>[2x]MATGRT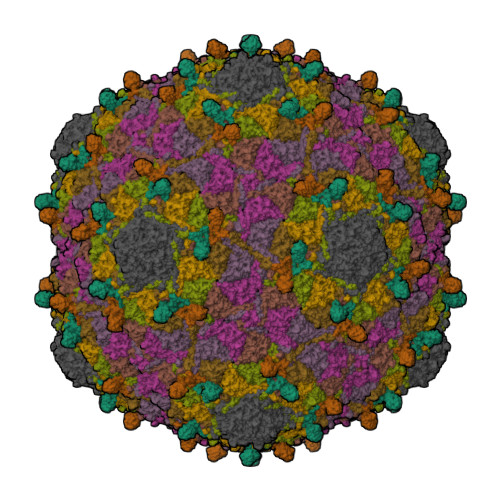TEGRTVTVTTASNTTITGAAGTFVASDVGRTITRAGIPAGTTITAVASGTSATISAAATTSATSAATLGSLNGQSQGLVGWSPETDTEAGAYSVAATNAGTVTPDRLTNAFTPVSQRGRG;>[7x]MGIYRKKDVIPIPYNNLTSRTDAQALIPEEVSKEMLGKATEQSAVLQQFRRIPVGRNQVRFPVLSALPVAYWVNGDTGLKQTTEINWTNKYLNIEEIATIVPVPDNVLADVDVNVWDEAMPYLIEAFGRTLDSAVVFGTNAPGTFPQAIVPAIAAAGNAVTEGSTAAQGGYLGDLDKAYGKVEEDGFEANGIIAGIGLKGKLRGARDANGQKIDPTRVGADLKSIDGLPVSYPMRGLWPSAGGAGTNVRALVGDWSQFVVGVRQDITLKVLDQAVIQDNTGAIIYNLAQQDMTALRLTFRVGWQVANTLNNDQPTEANRYPAASLIF Recently, a fluorophore named 5-((Z)-4-((2-hydroxyethyl)(methyl)amino)benzylidene)-3-methyl-2-((E)-styryl)-3,5-dihydro-4H-imidazol-4-one (NBSI), emitting in red spectrum, and its cognate aptamer named Clivia were identified, exhibiting a large Stokes shift. The overall structure uses a monomeric, non-G-quadruplex compact coaxial architecture, with NBSI sandwiched at the core junction. The overall structure of the complex adopts a coaxial long helix fold and is stabilized by continuous stacking interactions from the bottom stem P1 to the apical stem P2 with the ligand NBSI intercalated in the zipped junction region at the interface of stems P1 and P2. Our structural investigation of the Clivia aptamer bound to NBSI or NBSI derivatives revealed that the Clivia aptamer adopts a non-G-quadruplex scaffold supporting a specific ligand-binding pocket, suggesting a new fluorescence activation mechanism.

Two additional reported derivatives of NBSI, designated NBSI565 (3) and NBSI618 (4), were generated by introducing a 4-OH or 4-CN group to the styryl moiety of NBSI571, respectively. In NBSI618, a 4-CN group was incorporated into the styryl moiety and resulted in an excitation maximum at 510 nm and an emission maximum at 618 nm, thereby achieving a substantial Stokes shift of 108 nm. The distinct 3D fluorescence spectra of free NBSI618 in buffer and Clivia-bound NBSI618 clearly demonstrated that the binding of Clivia induced a notable change in the fluorescence properties of NBSI618, as evidenced by a shift in the excitation wavelength. Structure determination of the Clivia–NBSI618 complex revealed that NBSI618 retained the ligand conformation and interaction observed for NBSI, NBSI571 and NBSI565. The elongated 4-cyano-benzylidene moiety of NBSI618 was capsuled within the binding pocket of Clivia. Detailed analysis revealed a substantial increase in the buried area of the fluorophore within Clivia, expanding from 383.2 Å2 for NBSI571 to 412.1 Å2 for NBSI618. This enhancement highlights the robust ligand-binding pocket of the Clivia aptamer, potentially contributing to the remarkably large Stokes shift observed in NBSI derivatives.

>[2x]GGAAGAUUGUAAACAUGCCGAAAGGCAGACACUUCC> TSLREEEESQDNPFYFNSDNSWNTLFKNQYGHIRVLQRFDQQSKRLQNLEDYRLVEFRSKPETLLLPQQADAELLLVVRSGSAILVLVKPDDRREYFFLTSDNPIFSDHQKIPAGTIFYLVNPDPKEDLRIIQLAMPVNNPQIHEFFLS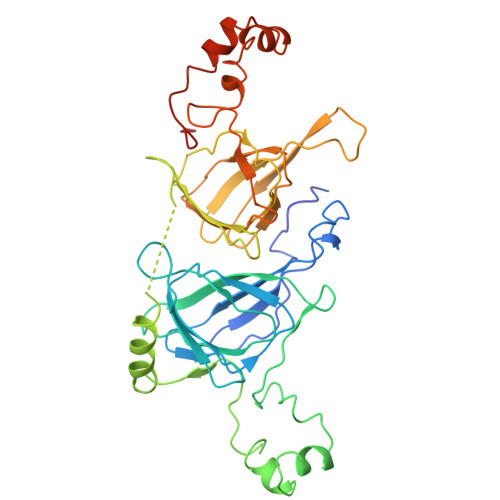STEAQQSYLQEFSKHILEASFNSKFEEINRVLFEEEGQQEGVIVNIDSEQIKELSKHAKSSSRKSLSKQDNTIGNEFGNLTERTDNSLNVLISSIEMEEGALFVPHYYSKAIVILVVNEGEAHVELVGPKGNKETLEYESYRAELSKDDVFVIPAAYPVAIKATSNVNFTGFGINANNNNRNLLAGKTDNVISSIGRALDGKDVLGLTFSGSGDEVMKLINKQSGSYFVDAHHHQQEQQKGRKGAFVY>MNNMNVIIADDHPIVLFGIRKSLEQIEWVNVVGEFEDSTALINNLPKLDAHVLITDLSMPGDKYGDGITLIKYIKRHFPSLSIIVLTMNNNPAILSAVLDLDIEGIVLKQGAPTDLPKALAALQKGKKFTPESVSRLLEKISAGGYGDKRLSPKESEVLRLFAEGFLVTEIAKKLNRSIKTISSQKKSAMMKLGVENDIALLNYLSSVTLSPADKD[2x]

At its core are three multidomain proteins, two hybrid histidine kinases (RcsC and RcsD) and a response regulator (RcsB). RcsB belongs to the FixJ/NarL family of response regulators with two domains connected by a long linker. The N-terminal REC (receiver) domain of RcsB is composed of a five-stranded central β-sheet surrounded by five α-helices and contains the conserved aspartyl residue (D56) that serves as the phosphoryl acceptor. The C-terminal DNA-binding domain (helix-turn-helix [HTH]) of RcsB has a four-helix bundle fold with a classical helix-turn-helix DNA recognition motif.

Here, we present crystal structures of unphosphorylated RcsB in complex with the consensus DNA-binding sequence of 22-mer (DNA22) and 18-mer (DNA18) of the flhDC operon from Escherichia coli determined at 3.15- and 3.37-Å resolution, respectively. The asymmetric unit of the RcsB crystal in complex with DNA22 contained one RcsB dimer bound to one double helix DNA, whereas the RcsB crystal in complex with DNA18 contained an RcsB tetramer (two RcsB dimers) bound to two parallel double helical DNAs. In both crystal forms, the RcsB dimers displayed similar structures, and the DNA had a classical B form with an average base pair rise and twist of 3.2 Å and 34°, respectively; the DNA was slightly bent along the surfaces of the RcsB HTH domains. The RcsB dimer observed in two different crystal forms is asymmetric. The subunits in the dimer were not related by a two-fold rotation axis of symmetry. Instead, an approximate two-fold axis was present between each of the RcsB domains of a dimer. However, these two axes met each other at an angle of about 120°. In the RcsB-DNA complex, the helices that form the HTH DNA recognition motif of the DNA-binding domain (α8 and α9) bound to the floor of the DNA major groove perpendicular to the DNA helical axis. K180 and S184, located on helix α9, made hydrogen bonds (H-bonds) with G-8, A−9 and A−6 in one-half-site (TTAGGAA) or with G−30, A−31, and A−28 in its complement (TCTAAGA) on the other half-site of the DNA. The side chain amino group of K192 in the RcsB-DNA22 complex contributes to electrostatic interactions, but it is too far away for a direct H-bond.>[2x]MSQRITIDPVTRIEGHLRIDCEIENGVVSKAWASGTMWRGMEEIVKNRDPRDAWMIVQRICGVCTTTHALSSVRAAESALNIDVPVNAQYIRNIILAAHTTHDHIVHFYQLSALDWVDITSALQADPTKASEMLKGVSTWHLNSPEEFTKVQNKIKDLVASGQLGIFANGYWGHPAMKLPPEVNLIAVAHYLQALECQRDANRVVALLGGKTPHIQNLAVGGVANPINLDGLGVLNLERLMYIKSFIDKLSDFVEQVYKVDTAVIAAFYPEWLTRGKGAV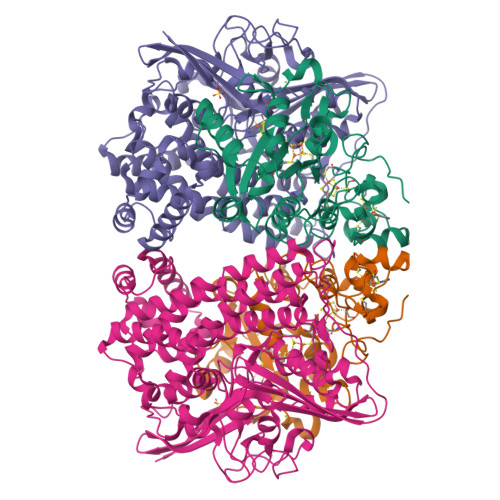NYLSVPEFPTDSKNGSFLFPGGYIENADLSSYRPITSHSDEYLIKGIQESAKHSWYKDEAPQAPWEGTTIPAYDGWSDDGKYSWVKSPTFYGKTVEVGPLANMLVKLAAGRESTQNKLNEIVAIYQKLTGNTLEVAQLHSTLGRIIGRTVHCCELQDILQNQYSALITNIGKGDHTTFVKPNIPATGEFKGVGFLEAPRGMLSHWMVIKDGIISNYQAVVPSTWNSGPRNFNDDVGPYEQSLVGTPVADPNKPLEVVRTIHSFDPCMACAVHVVDADGNEVVSVKVL;>[2x]MAESVTNPQRPPVIWIGAQECTGCTESLLRATHPTVENLVLETISLEYHEVLSAAFGHQVEENKHNALEKYKGQYVLVVDGSIPLKDNGIYCMVAGEPIVDHIRKAAEGAAAIIAIGSCSAWGGVAAAGVNPTGAVSLQEVLPGKTVINIPGCPPNPHNFLATVAHIITYGKPPKLDDKNRPTFAYGRLIHEHCERRPHFDAGRFAKEFGDEGHREGWCLYHLGCKGPETYGNCSTLQFCDVGGVWPVAIGHPCYGCNEEGIGFHKGIHQLANVENQTPRSQKPDVNAKEGGHHHHHH>[2x]GSKKHTGYVGLKNQGATCYMNSLLQTLFFTNQLRKAVYMMPTEGDDSSKSVPLALQRVFYELQHSDKPVGTKKLTKSFGWETLDSFMQHDVQELCRVLLDNVENKMKGTCVEGTIPKLFRGKMVSYIQCKEVDYRSDRREDYYDIQLSIKGKKNIFESFVDYVAVEQLDGDNKYDAGEHGLQEAEKGVKFLTLPP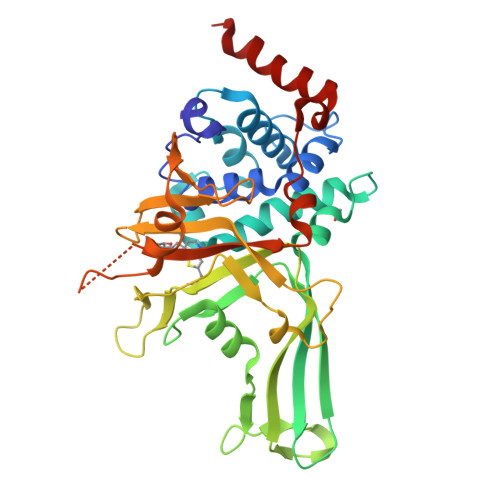VLHLQLMRFMYDPQTDQNIKINDRFEFPEQLPLDEFLQKTDPKDPANYILHAVLVHSGDNHGGHYVVYLNPKGDGKWCKFDDDVVSRCTKEEAIEHNYGGHDDDLSVRHCTNAYMLVYIRESKLSEVLQAVTDHDIPQQLVERLQEEKRIEAQKR>[3x]QGSCMSITINPSRPSVNNIGQVDIDSVILGRPGAIGS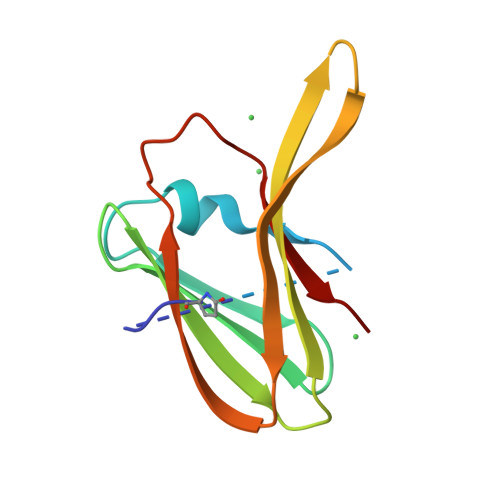WELNNFITIGLNRVNADTVRVNIRNTGRTNRLIITQWDNTVTRGDVYELFGDYALIQGRGSFCLNIRSDTGRENWRMQLEN Baculovirus Autographa californica multiple nucleopolyhedrovirus (AcMNPV) has been widely used as a bioinsecticide and a protein expression vector. The DNA genome, along with the baculovirus basic DNA-binding protein P6.9 protein, is encapsulated by an enveloped, rod-shaped nucleocapsid; the major capsid protein VP39 and some additional minor proteins are known to comprise the nucleocapsid. Here, we show a 3.2 Å resolution structure of helical cylindrical body of the AcMNPV nucleocapsid, composed of VP39, as well as 4.3 Å resolution structures of both the head and the base of the nucleocapsid composed of over 100 protein subunits. Surprisingly, the C14 symmetric base had nearly identical features to that of the apical head, except for that in the central regions. Both the head and base could be further segmented into three parts: an outer shell, an inner layer and a central region.

Local refinement of the main helical cylinder in the AcMNPV capsid resulted in a 3.2 Å resolution map for the major capsid protein, which was sufficient to build a de novo atomic model for VP39 directly from the density map. The asymmetric unit of the helical cylinder is parallelogram-shaped, containing a VP39 dimer (VP39A and VP39B) with local 2-fold symmetry. Asymmetric units, which contain two VP39s, are related to each other by a rotation of ~18.5° about the helical axis and a rise of 44.1 Å along the helical axis, generating a right-handed, 14-start helix. The major capsid protein of AcMNPV, VP39, has several common elements to that of the HK97-like fold, including the E-loop linking a two-stranded anti-parallel β-sheet, a long “spine helix” in P-domain, and a distinct four-stranded anti-parallel β-sheet in the A-domain. In contrast to other dsDNA viruses where the HK97-like fold is organized with icosahedral symmetry, VP39, with its HK97-like fold protein, is found, for the first time, to be organized with helical symmetry in baculovirus. At the center of the VP39 dimer, cysteines (Cys229) from each VP39 form a disulfide bond. Residues Asn270-Pro296 in the C-terminal region, in addition to Tyr250, form a ring-like structure, creating a “hole” for the insertion of the “E-loop” from the adjacent VP39. When taken together with the intra-asymmetric unit knot, the C-terminals of VP39 form a series of continuous interactions with an “S”-like shape, linking the neighboring helical starts together. In addition to Cys229, which forms a disulfide bond between the two VP39s in each asymmetric unit, Cys29, Cys169 and Cys132 can form disulfide bonds between VP39s from adjacent asymmetric units. These disulfide bonds lock the neighboring dimers together and are likely critical contributors in the assembly and stability of the helical capsid cylinder.

>[2x]MALVPVGMAPRQMRVNRCIFASIVSFDACITYKSPCSPDAYHDDGWFICNNHLIKRFKMSKMVLPIFDEDDNQFKMTIARHLVGNKERGIKRILIPSATNYQDVFNLNSMMQAEQLIFHLIYNNENAVNTICDNLKYTEGFTSNTQRVIHSVYATTKSILDTTNPNTFCSRVSRDELRFFDVTNARALRGGAGDQLFNNYSGFLQNLIRRAVAPEYLQIDTEELRFRNCATCIIDETGLVASVPDGPELYNPIRSSDIMRSQPNRLQIRNVLKFEGDTRELDRTLSGYEEYPTYVPLFLGYQIINSENNFLRNDFIPRANPNATLGGGAVAGPAPGVAGEAGGGIAV>[6x]TSSVAAFTSGTIG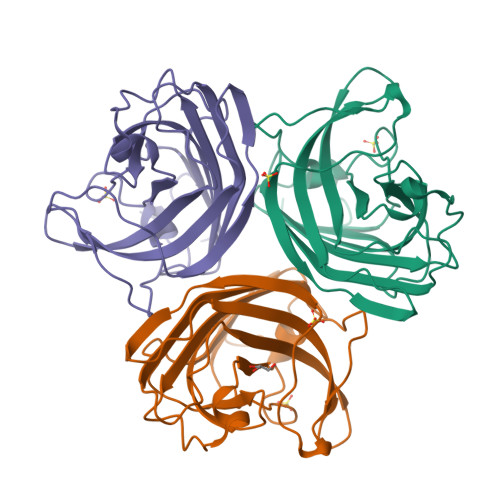LSSPTGNFVSSSNNPFNGSYFLQQINTMGMLTTSLYVKVDTTTMGTRPTGAVNENARYFTVWVSSFLTQCNPSNIGQGTLEPSNISMTSFEPARNPISPPVFNMNQNIPYYASRFGVLESYRPIFTGSLNTGSIDVRMQVTPVLATNNTTYNLIAFTFQCASAGLFNPTVNGTVAIGPVVHTCPAARAPVTV>[4x]MYCLYERPINSKTGVLEWNGD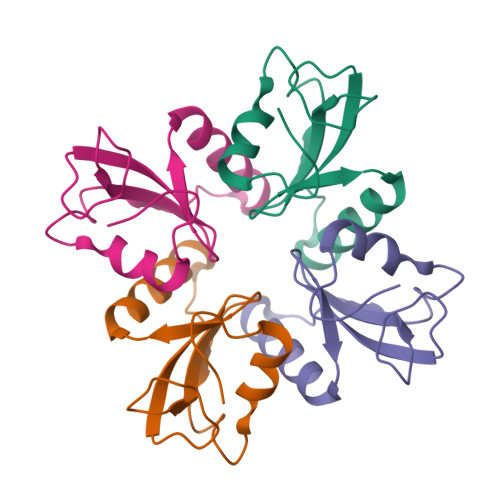AWTVMFCNGVNCRRVSHPDEMKVIEDIYRKNNGKDIPFYSQKEWNKNAPWYNRLETVCPVVGITKKS>GEDEIESAGVSASEVESSATKQKVALHPHDLDERIPGLADLHNQTLGDPQITIVIIDGDPDYTLSCFEGAEVSKVFPYWHEPAEPITPEDYAAFQSIRDQGLKGKEKEEALEAVIPDTKDRIVLNDHACHVTSTIVGQEHSPVFGIAPNCRVINMPQDAVIRGNYDDVMS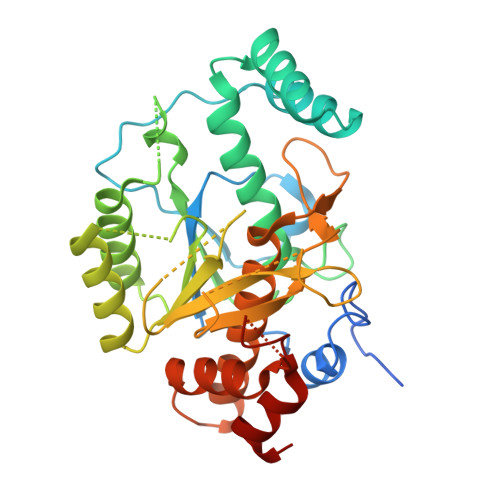PLNLARAIDLALELGANIIHCAFCRPTQTSEGEEILVQAIKKCQDNNVLIVSPTGNNSNESWCLPAVLPGTLAVGAAKVDGTPCHFSNWGGNNTKEGILAPGEEILGAQPCTEEPVRLTGTSMAAPVMTGISALLMSLQVQQGKPVDAEAVRTALLKTAIPCDPEVVEEPERCLRGFVNIPGAMKVLFGQ[2x]>[4x]SHMSGLKPCVDWLQVTFKTGQDSVKKCVEKLEKVFEILGLNEAEFLPLKNGKYGYKQGVAFQGNPVLAVYYDGADDMGIHVEMTGQGCRLFELHTSINWYELFYRLVYEYEVNITRLDVAVDDFKGYFKINTLVKKLKDDEVTSRFKKARHIENIVIEGGETIGHTLYFGAPSSDIQVRFYEKNVQMGMDIDVWNRTEIQLRDDRAHVVAQIIADDVLPLGEIVAGLLRNYIQFRTRKATDKNKKRWPLARFWLNFLGDVQPLRIAKQMPK

In Gram-positive organisms, the smaller plasmids often replicate via a rolling circle mechanism, a process mediated by a multi-functional replication initiation protein (Rep) encoded on that plasmid. The Rep proteins possess two related catalytic activities, a type-I topoisomerase-like cleavage activity in which they form a nick in the (+) strand at the origin of replication to initiate DNA synthesis, and a religation activity to join the ends of the parental strand that is displaced during replication. Despite low overall sequence identity, there is a high degree of structural conservation between the catalytic domains of the Rep proteins from these Geobacillus stearothermophilus and Staphylococcus aureus plasmids. Structure-based sequence alignment reveals the conserved residues are almost exclusively located in the β-strands containing the Rep_trans motifs, and it is likely the crescent-shaped catalytic domain represents the canonical fold for the Rep_trans protein family.

In this report we describe the structure determination of the core domain of replication initiator protein of cryptic plasmid pSTK1 (25,26) from Geobacillus stearothermophilus (RepSTK1 residues 1–269 (27), hereafter referred to as RepSTK1). RepSTK1 formed crystals belonging to space-group P212121 with four molecules per asymmetric unit, arranged as two dimers. The structure was determined to a resolution of 2.3 Å by MIRAS phasing using mercury chloride and potassium chloroplatinate derivatives. Each subunit is crescent shaped, with a concave inner surface formed by a 10-stranded, antiparallel β-sheet the outer surface of which is decorated with eight α-helices. The subunits interact via interfaces at either end of the crescent to form a ring where the diameter of the central cavity is 20 Å. The model of RepSTK1, crystallized in the absence of divalent metal ions, contains a water molecule in the metal binding site. The interior cavity of the catalytic domains is also positively charged, when calculated with a divalent metal ion modelled into the active site. The DNA binding residues of RepSTK1 have not been identified, but two extended loops protrude from the surface of the protein (the top of the protein as shown in Figures 2A and 5C) replacing the separate DBD found in the staphylococcal proteins. The differing quaternary structures of the catalytic domains of the Rep proteins may represent functionally relevant conformations, since the active site lies on the inner surface of the β-sheet and the diameter of the central cavity of RepSTK1 would severely hinder access of the dsDNA substrate. Enabling RepSTK1 to undergo such a conformational change would require disruption of one of the interfaces stabilising the ring, with the smaller of the two interfaces needing significantly less energy to disrupt.> MGSSHHHHHHMSRLSEPSPYVEFDRRQWRALRMSTPLALTEEELVGLRGLGEQIDLLEVEEVYLPLARLIHLQVAARQRLFAATAEFLGEPQQNPDRPVPFIIGVAGSVAVGKSTTARVLQALLARWDHHPRVDLVTTDGFLYPNAELQRRNLMHRKGFPESYNRRALMRFVTSVKSGSDYACAPVYSHLHYDIIPGAEQVVRHPDILILEGLNVLQTGPTLMVSDLFDFSLYVDARIEDIEQWYVSRFLAMRTTAFADP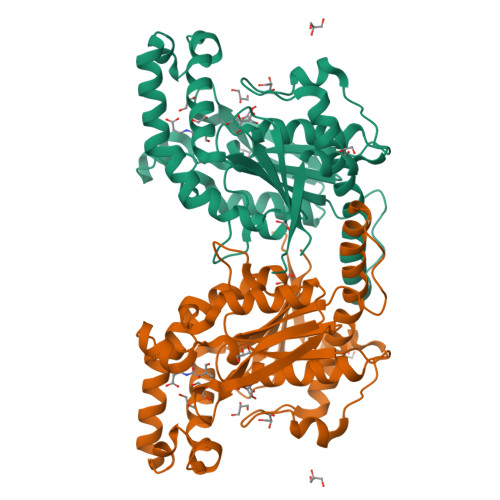ESHFHHYAAFSDSQAVVAAREIWRTINRPNLVENILPTRPRATLVLRKDADHSINRLRLRKL> MLPRETDEEPEEPGRRGSFVEMVDNLRGKSGQGYYVEMTVGSPPQTLNILVDTGSSNFAVGAAPHPFLHRYYQRQLSSTYRDLRKGVYVPYTQGKWEGELGTDLVSIPHGPNVTVRANIAAIT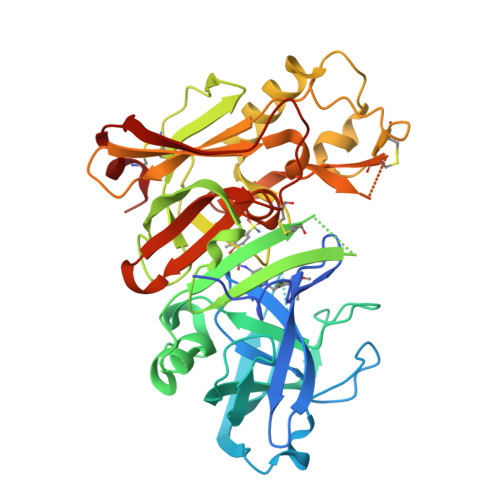ESDKFFINGSNWEGILGLAYAEIARPDDSLEPFFDSLVKQTHVPNLFSLQLCGAGFPLNQSEVLASVGGSMIIGGIDHSLYTGSLWYTPIRREWYYEVIIVRVEINGQDLKMDCKEYNYDKSIVDSGTTNLRLPKKVFEAAVKSIKAASSTEKFPDGFWLGEQLVCWQAGTTPWNIFPVISLYLMGEVTNQSFRITILPQQYLRPVEDVATSQDDCYKFAISQSSTGTVMGAVIMEGFYVVFDRARKRIGFAVSACHVHDEFRTAAVEGPFVTLDMEDCGYN>RILPEVKVEGELGGSVTIKCPLPEMHVRIYLCREMAGSGTCGTVVSTTNFIKAEYKGRVTLKQYPRKNLFLVEVTQLTESDSGVYACGAGMNTDRGKTQKVTLNVHSEYEPSWEEQPMPETPKWFHLPYLFQMPAYASSSKFVTRVTTPAQRGKVPPVHHSSPTTQITHRPRVSRASSVAGDKPRTFLPSTTASKISALEGLLKPQTPSYNHHTRLHRQRALDYGSQSGREGQG[2x];>IAELPPKVSVFVPPRDGFFGNPRKSKLICQATGFSPRQIQVSWLREGKQVGSGVTTDQVQAEAKESGPTTYKVTSTLTIKESDWLGQSMFTCRVDHRGLTFQQNASSMCVPDQDTAIRVFAIPPSFASIFLTKSTKLTCLVTDLTTYDSVTISWTRQNGEAVKTHTNISESHPNATFSAVGEASICEDDWNSGERFTCTVTHTDLPSPLKQTISRPKGVALHRPDVYLLPPAREQLNLRESATITCLVTGFSPADVFVQWMQRGQPLSPEKYVTSAPMPEPQAPGRYFAHSILTVSEEEWNTGETYTCVVAHEALPNRVTERTVDKSTGKPTLYNVSLVMSDTAGTCY[4x]

FcμR is the IgM antibody isotype-specific Fc receptor involved in the survival and activation of B cells. In this study, we image a complex of the ectodomain of human FcμR and the IgM-Fc pentameric core using single-particle cryogenic electron microscopy (cryo-EM). The analysis reveals multiple binding sites for the N-terminal Ig domain of FcμR on the Cμ4 domain dimers within the IgM constant region and provides a framework for understanding FcμR’s role in immunoglobulin recognition and signalling. A key common feature of the FcμR binding sites is that only the Cμ4 domains are involved in the interactions.

Two binding sites (position 1f and 3f) which have highest occupancies of FcμR, reached high-resolution (3.5 Å and 3.1 Å) in the cryo-EM maps, thus allowing the atomic model interpretation of the FcμR Ig-like domain and the IgM binding interface. Due to the quasi six-fold symmetry within the Cμ4 domains in IgM pentamer, the FcμR molecules at position 1f and 3f share almost identical interactions with the two Cμ4 domains (Cμ4-A and Cμ4-B) in subunits Fcμ1 and Fcμ3 respectively. The Cμ4-B chain of the IgM subunit (grey in Fig. 4b) contains a central hub of residues (Asn465-Glu468) for FcμR binding, which interacts with all three CDR loops on FcμR including CDR1 (Arg45), CDR2 (Thr60/Ser63/Thr65) and CDR3 (Thr110/Asp111). CDR2 of FcμR forms additional interactions including Lys69, which form a hydrogen bond with Glu526 on Cμ4-B chain and Asn66, which contacts neighbouring Cμ4-A chain (Gln510 and Arg514). In addition to the common features, different interactions between FcμR and binding sites at subunits Fcμ1 and Fcμ3 result from the asymmetrical structure of IgM pentamer. At position 3f, Arg112 in FcμR interacts with two carbonyl groups (Thr530 and Gly531) on the Cμ4-2B domain in the neighbouring IgM subunit, which is presumably shared by all the FcμR bound at internal subunits (subunits Fcμ2-4). Furthermore, additional contact from the carbohydrate chain extending from Asn563 on the tailpiece towards the FcμR is observed at subunit Fcμ3. Interestingly, although all ten Asn563 sites are glycosylated, only the carbohydrates at subunit Fcμ3 are involved in FcμR engagement. This is due to the mismatch between the quasi six-fold symmetrical FcμR binding sites and the two-fold symmetrical IgM tailpiece where Asn563 is located, resulting in different relative positions between the glycosylation sites and FcμR molecules at different subunits.>MAHHHHHHMQIIHTIRELRTWRENTGKVAFVPTMGNLHEGHLAL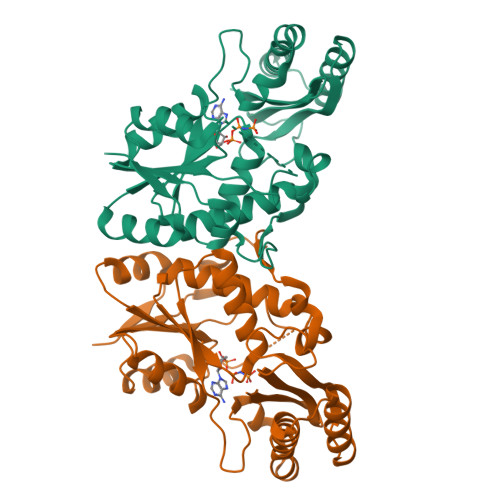VREARKRADNVVVSIFVNRLQFGQGEDFDKYPRTLQQDADKLAAEGVAVVFAPDEKELYPNVEQRYNVEPPHLQNELCGKFRPGHFRGVATVVSKLFNIVLPDVACFGKKDYQQLAVIKGLTEDLNFDIEIVPVDTGRAADGLALSSRNRYLSVGERAEAPRLYRELQAVAESLKQGGLDYAGLERQAADHLTAAGWLVDYVEIRRADTLEMARAGDKKLVVLAAARLGTTRLIDNVEVGLP[2x]>MWQQAIGDALGITARNLKKFGDRFPHVSDGSNKYVLNDNTDWTDGFWSGILWLCYEYTGDEQYREGAVRTVASFRERLDRFENLDHHNIGFLYSLSAKAQWIVEKDESARKLALDAADVLMRRWRADAGIIQAWGPKGDPENGGRIIIDCLLNLPLLLWAGEQTGDPEYRRVAEAHALKSRRFLVRGDDSSYHTFYFDPENGNAIRGGTHQ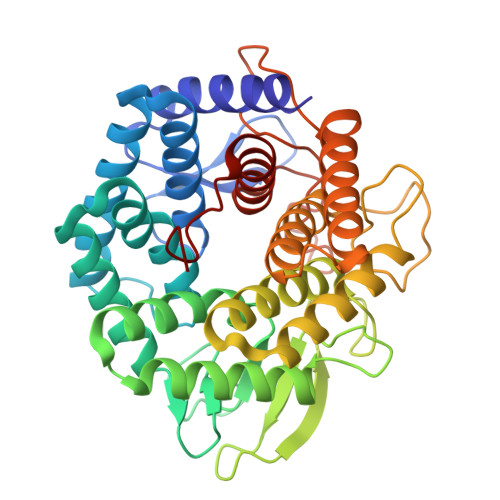GNTDGSTWTRGQAWGIYGFALNSRYLGNADLLETAKRMARHFLARVPEDGVVYWDFEVPQEPSSYRDSSASAITACGLLEIASQLDESDPERQRFIDAAKTTVTALRDGYAERDDGEAEGFIRRGSYHVRGGISPDDYTIWGDYYYLEALLRLERGVTGYWYERGR[2x]>[2x]MRRHYRDLIRNTPMPDTPQDIADLRALLDEDEAEMSVVFSDPSQPDNPIIYVSDAFLVQTGYTLEEVLGRNCRFLQGPDTNPHAVEAIRQGLKAETRFTIDILN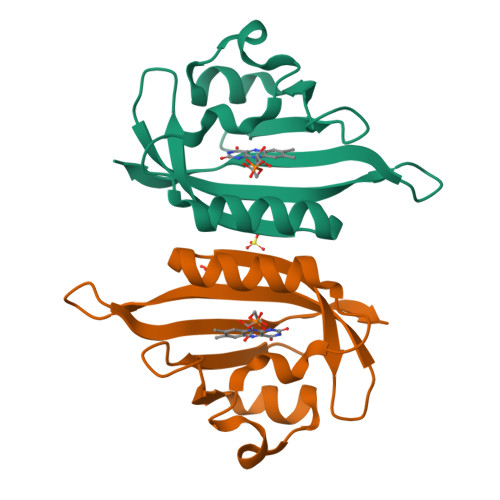YRKDGSAFVNRLRIRPIYDPEGNLMFFAGAQNPVLEHHHHHH> TMGGDALRVPFLDFATATPKRHQTVVPGVGTLHDCCEHSPLFSAVARRLLFNSLVPAQLKGRDFGGDHTAKLEFLAPELVRAVARLRFKECAPADVVPQRNAYYSVLNTFQALHRSEAFRQLVHFVRDFAQLLKTSFRASSLTETTGPPKKRAKVDVATHGRTYGTLELFQKMILMHATYFLAAVLLGDHAEQVNTFLRLVFEIPLFSDAAVRHFRQRATVFLVPRRHGKTWFLVPLIALSLASFRGIKIGYTAHIRKATEPVFEEIDACLRGWFGSARVDHVKGETISFSFPDGSRSTIVFASSHNTNGIRGQDFNLLFVDEANFIRPDAVQTIMGFLNQANCKIIFVSSTNTGKASTSFLYNLRGAADELLNVVTYICDDHMPRVVTHTNATACSCYILNKPVFITMDGAVRRTADLFLADSFMQEIIGGQARETGDDRPVLTKSAGERFLLYRPSTTTNSGLMAPDLYVYVDPAFTANTRASGTGVAVVGRYRDDYIIFALEHFFLRALTGSAPADIARCVVHSLTQVLALHPGAFRGVRVAVEGNSSQDSAVAIATHVHTEMHRLLASEGADAGSGPELLFYHCEPPGSAVLYPFFLLNKQKTPAFEHFIKKFNSGGVMASQEIVSATVRLQTDPVEYLLEQLNNL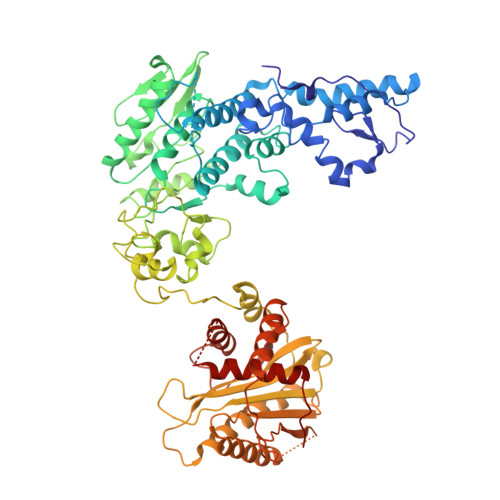TETVSPNTDVRTYSGKRNGASDDLMVAVIMAIYLAAQAGPPHT2-amino-7-(4,4-difluorocyclohexyl)-5-oxo-5H-[1]benzopyrano[2,3-b]pyridine-3-carboxylic acid | C19 H16 F2 N2 O4 | 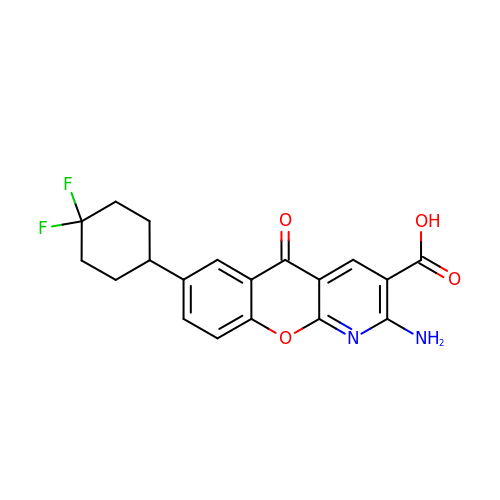YBTHXDAXRWKGKS-UHFFFAOYSA-N>[8x]GPLGSDADKNDPAGKDQQVNVGETPKAEDSIGNLPDLPKGTTVAFETPVDTATPGDKPAKVVVTYPDGSKDTVDVTVKVVDPRTDADKNDPAGKDQQVNVGETPKAEDSIGNLPDLPKGTTVAFETPVDTATPGDKPAKVVVTYPDGSKDTVDVTVKVVDPRT

Proteins attached to the surface of group A and group B streptococcal human pathogens that contain tandemly arrayed Rib domains have been associated with invasive infections and proposed as potential vaccine candidates. Here, we study Rib domains from Rib, R28, and from a surface protein from Lactobacillus acidophilus. Together, these 5 structures of homologous Rib domains, and further sequence analyses, show Rib is an example of domain atrophy, a rare event in domain structural evolution involving the loss of core secondary structure elements, and also reveal the remarkable structural malleability of this domain family. The structure, molecular dynamics simulations, and small angle X-ray scattering of a Rib domain pair suggest tandemly arrayed domains are likely to form an elongated rod on the bacterial cell surface, thus suggesting a possible mechanism of immune evasion mediated through domain number variation.

Rib domains are often found tandemly arrayed; thus, to examine the interdomain orientation, the structure of a 2-domain Rib construct (Rib2R) (residues 230 to 387) was solved. The interdomain linker is short and consists of the residues DPRT. The similarity of the Tm of RibR and Rib2R is consistent with the lack of a large stabilizing interdomain interface. Importantly, both particles display very similar RgC values (8.7 Å, RibR; 8.5 Å, Rib2R), suggesting that Rib2R forms an elongated molecule represented by 2 RibR molecules stacked end-on-end. To further assess the interdomain orientation, we performed molecular dynamics (MD) simulations of fully solvated Rib2R at room temperature (303 K). The rmsd from the crystal structure fluctuates by up to 10 Å while that of the individual domains varies by ∼2 Å, showing that the mutual arrangement of the domains fluctuates in time around the crystal structure. Remarkably, the 2-domain structure remains extended on average, with an end-to-end distance of 96.2 ± 9.5 Å, which is consistent with both the Dmax calculated from SAXS (97 Å) and the length of the crystal structure (98 Å). Modeling of the 3 interdomain rotation angles suggests that, while a wide range of long axis (x) rotations (α) are accommodated, rotations around the y and z axes (β, γ) occupy a more narrow distribution. Given the lack of interdomain stabilization in Rib2R, rigidity in the interdomain linker is likely to be influential in maintaining the interdomain interface. The most common linker length between tandem Rib domains is shorter at just 2 residues, which suggests that most tandem Rib domains will be more constrained than in Rib2R and thus are likely to also form relatively rigid, extended arrays.>[6x]AQYEDGKQYTTLEKPVAGAPQVLEFFSFFCPHCYQFEEVLHISDNVKKKLPEGVKMTKYHVNFMGGDLGKDLTQAWAVAMALGVEDKVTVPLFE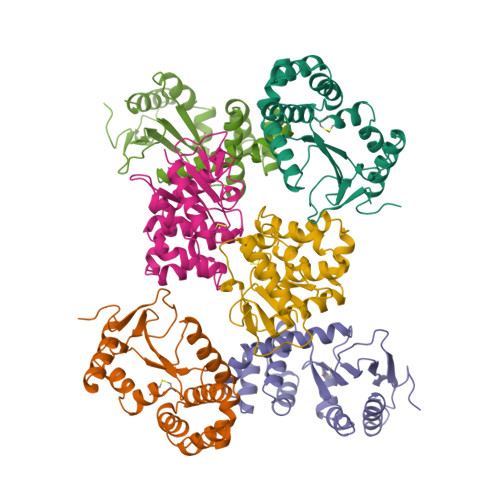GVQKTQTIRSASDIRDVFINAGIKGEEYDAAWNSFVVKSLVAQQEKAAADVQLRGVAAMFVNGKYQLNPQGMDTSNMDVFVQQYADTVKYLSEKK2-chlorobenzyl carbamimidothioate | C8 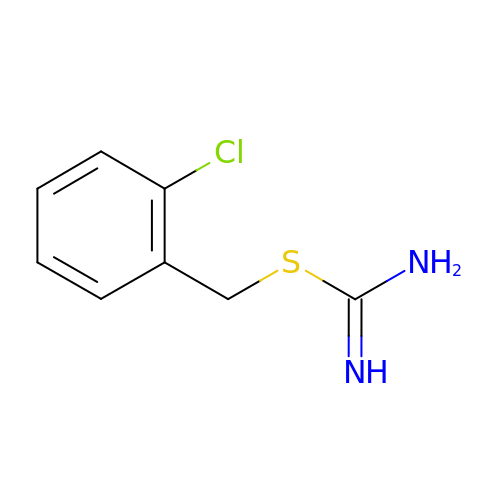H9 Cl N2 S | SFKYKNIIEFCNBX-UHFFFAOYSA-N>[6x]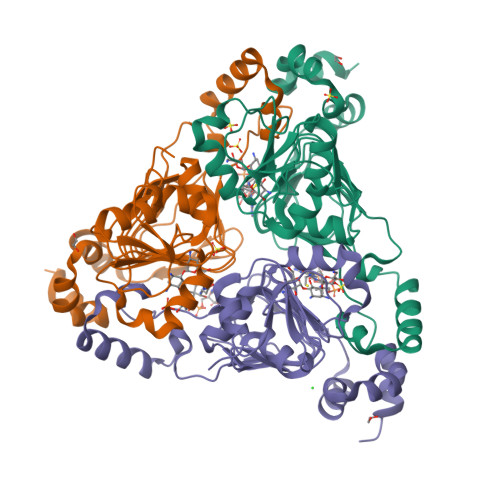QGMKTRLEQVLERYLNGREVAVWGVPTRRLLRALKPFKFHTADRVDPQYHYVVAVTDDDLTDFLSDEQSKSFQYANDYLTFDDEGGELPFERMCFNVPVGRQTYFGDGVVGACENGYIKSIGQFTSINGTAEIHANHQLNMTFVSDDIQNFFNEESMAVFQEKLRKDPKHPYAYSKEPMTIGSDVYIGAHAFINASTVTSIGDGAIIGSGAVVLENVPPFAVVVGVPARIKRYRFSKEMIETLLRVKWWDWSIEEINENVDALISPELFMKKYGSL>MGSDKIHHHHHHMTENSRKTATELFEFLDGLGISHTTKQHEPVFTVAESQSLRDLIPGGHTKNLFVKDKKDQYFVLTVEENAVVDLKSVHKTIGAASRVSFGRPEKMLEYLGVVPGSVTVFGAINDTARQV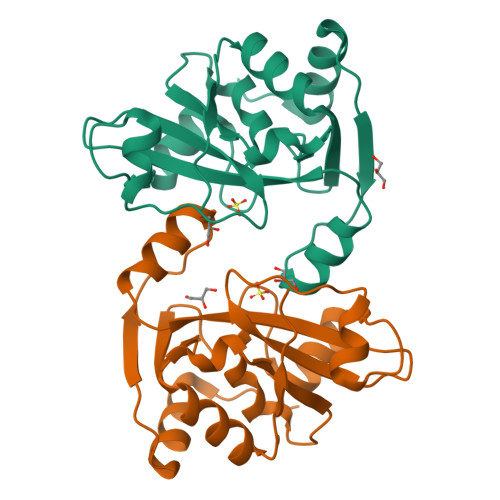TFVLDSDLLENELVNGHPLSNDQTTTIASKDLIRFLEATGHAPLVLKVSE[2x]Protein tyrosine phosphorylation regulates the production of capsular polysaccharide, an essential virulence factor of the deadly pathogen Vibrio vulnificus. The process requires the protein tyrosine kinase Wzc and its cognate phosphatase Wzb, both of which are largely uncharacterized. VvWzb belongs to the low-molecular-weight protein tyrosine phosphatase (LMWPTP) family. Interestingly, it contains an extra four-residue insertion in the W-loop, distinct from all known LMWPTPs.

In the presence of benzylphosphonate, a compound that mimics the phenylphosphate moiety of the substrate phosphotyrosine, VvWzb and VvWzbC9A crystallized in space groups P1 and P212121, respectively. We were able to model one benzylphosphonate molecule (with occupancy of 1 and B-factor of 82.8, 142.8, 109.6, or 89.9 Å2) for each of the four protein chains in the wild-type (WT) structure. In VvWzb-benzylphosphonate complex, the substrate-mimicking benzylphosphonate is located at the bottom of the active site crevice. Its phosphonate group forms an extensive hydrogen-bonding network with the P-loop, including the main chain amide groups of the residues Val10, Gly11, Asn12, Ile13, Cys14, and Arg15, as well as the sulfhydryl group of Cys9 and the side-chain guanidine group of Arg15. The benzyl group of benzylphosphonate is flanked by residues Val10 of the P-loop and Tyr121 of the D-loop and further stabilized by Leu44 of the W-loop and Ile13 of the P-loop via hydrophobic interactions. Compared with the free structure, the W-loop undergoes a dramatic conformational rearrangement from an open to a closed conformation. Consequently, Glu40 is no longer oriented toward the active site cavity but turns outside. Instead, side chains of Ser42 and Leu44 turn to face the active site, forming the W-loop wall. In addition, side chains of Asp119 and Tyr121 of the D-loop also made small local conformational changes to interact with the ligand. All these conformational changes significantly reconfigure the active site crevice, which is narrower and deeper in shape as well as more positively charged compared with that of free VvWzb.

>GAMGFNKILVVCVGNICRSPTGERVLQKLLPNKTVASAGIAAEKSRLIGKPADAMAIEVAKENCVDVENHQSQQLTSALCSQYDLILVMEKGHMEALTQIAPEARGKTMLFGQWIGQKDIPDPYRQSKEAFVHAYQLIDEAAQAWAKKL[4x]ADP-ribosyl-acceptor hydrolase 3 (ARH3) cleaves PAR and mono(ADP-ribosyl)ation at serine following DNA damage. In contrast, ARH3 has a unique ARH fold and a di-Mg2+-containing catalytic center and can efficiently reverse not only PARylation but also mono(ADP-ribosyl)ation (MARylation) at serine; ARH3 can also cleave O-acetyl-ADPR and α-NAD+ in a Mg2+-dependent manner releasing free ADPR. While coordination of two magnesium ions (MgA and MgB) significantly enhances its catalytic efficiency, calcium binding suppresses its function. In the active site of ARH3, acidic residues, including Asp77, Asp78, Asp314, and Asp316, maintain the integrity of the bimetallic center and render the ideal alignment of the substrate for catalysis.

To test this model and dissect the structural basis for the inhibitory effect of Ca2+, we determined the structure of full-length ARH3 in complex with ADPR and Ca2+ at a resolution of 1.75 Å. Two metal ions (CaA and CaB) and ADPR are positioned in a way similar to those found in the Mg2+-bound form. Unlike the Mg2+-bound form where both Mg2+ ions have a similar octahedral coordination geometry with six ligands, the coordination architecture of CaA and CaB shows a notable difference. CaB is coordinated with a total of seven ligands with an average metal–ligand distance of 2.49 Å. In contrast, CaA shows an octahedral but highly relaxed geometry. In the ARH3–ADPR–Ca2+ complex, the orientation of 1″-OH group of the terminal ribose, corresponding to the 1″-O-linkage in uncleaved substrates, is tilted toward CaB. With respect to the Mg2+-bound form, the 1″-OH group is rotated ∼10° in the Ca2+-bound form. As a result, the 1″-OH group is directly coordinated to CaB, whereas 2″-OH bridges the dimetallic center by interacting with both Ca2+ ions. Notably, the metal-bridging water (μ-aqua) is missing in the Ca2+-bound form. Taken together, our findings suggest that the distorted di-Ca2+ metal center and the tilted conformation of 1″-OH, a position for the scissile O-linkage in substrates, are likely to interfere with a precise alignment of substrates for nucleophilic attack, resulting in suppression of enzymatic activities of ARH3.

>[4x]GPHMAAAAMAAAAGGGAGAARSLSRFRGCLAGALLGDCVGSFYEAHDTVDLTSVLRHVQSLEPDPGTPGSERTEALYYTDDTAMARALVQSLLAKEAFDEVDMAHRFAQEYKKDPDRGYGAGVVTVFKKLLNPKCRDVFEPARAQFNGKGSYGNGGAMRVAGISLAYSSVQDVQKFARLSAQLTHASSLGYNGAILQALAVHLALQGESSSEHFLKQLLGHMEDLEGDAQSVLDARELGMEERPYSSRLKKIGELLDQASVTREEVVSELGNGIAAFESVPTAIYCFLRCMEPDPEIPSAFNSLQRTLIYSISLGGDTDTIATMAGAIAGAYYGMDQVPESWQQSCEGYEETDILAQSLHRVFQKS>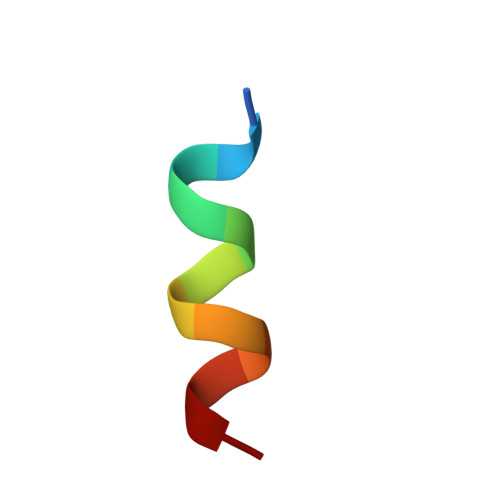 KYKKALKKLAKL>[2x]PNSLDQIDLLSTKSFPPCMRQLHKALRENHHLRHGGRMQYGLFLKGIGLTLEQALQFWKQEFIKGKMDPDKFD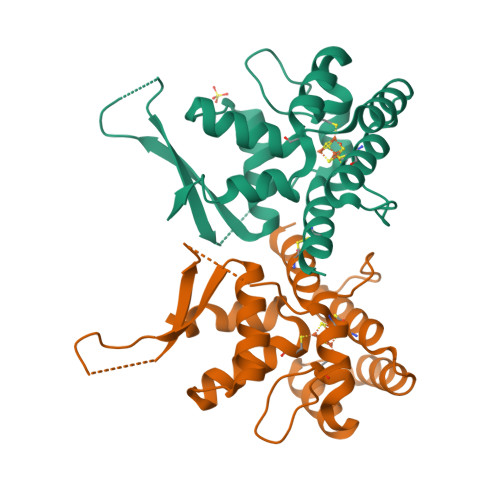KGFSYNIRHSFGKEGKRTDYTPFSCLKIILSNPPSQGDYHGCPFRHSDPELLKQKLQSYKISPGGISQILDLVKGTHYQVACQKYFEMIHNVDDCGFSLNHPNQFFCESQRILNG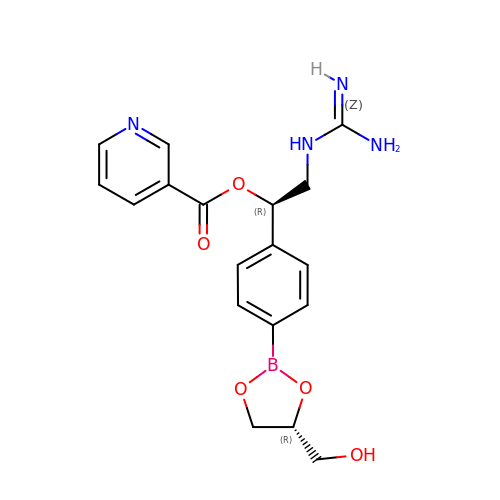(1R)-2-{[AMINO(IMINO)METHYL]AMINO}-1-{4-[(4R)-4-(HYDROXYMETHYL)-1,3,2-DIOXABOROLAN-2-YL]PHENYL}ETHYL NICOTINATE | C18 H21 B N4 O5 | HGLWHYRZHMOCMC-CVEARBPZSA-N> ISGGDAIYSSTGRCSLGFNVRSGSTYYFLTAGHCTDGATTWWANSARTTVL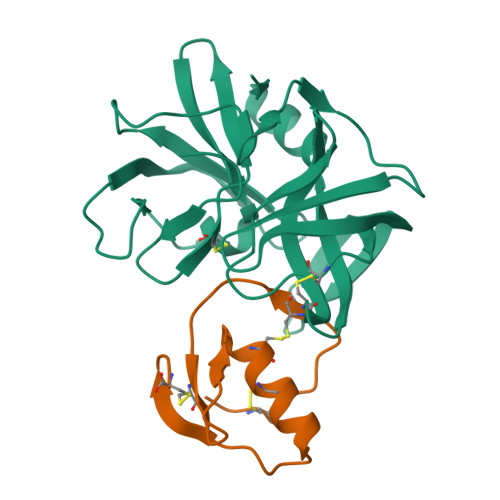GTTSGSSFPNNDYGIVRYTNTTIPKDGTVGGQDITSAANATVGMAVTRRGSTTGTHSGSVTALNATVNYGGGDVVYGMIRTNVCAEPGDSGGPLYSGTRAIGLTSGGSGNCSSGGTTFFQPVTEALSAYGVSVY;> VDCSEYPKPACTREYRPLCGSDNKTYGNKCNFCNAVVESNGTLTLSHFGKC> TSELRICRINKE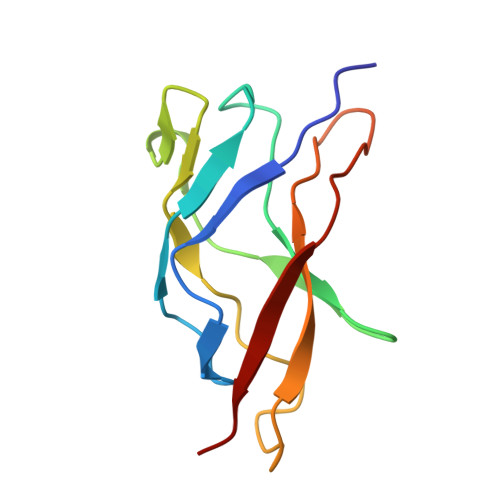SGPCTGGEELYLLCDKVQKEDISVVFSTASWEGRADFSQADVHRQIAIVFKTPPYEDLEISEPVTVNVFLQRLTDGVCSEPLPFTYLPR> MRVEGAIGKTPVVRLAKVVEPDMAEVWVKLEGLNPGGSIKDRPAWYMIKDAEERGILRPGSGQVIVEPTSGNTGIGLAMIA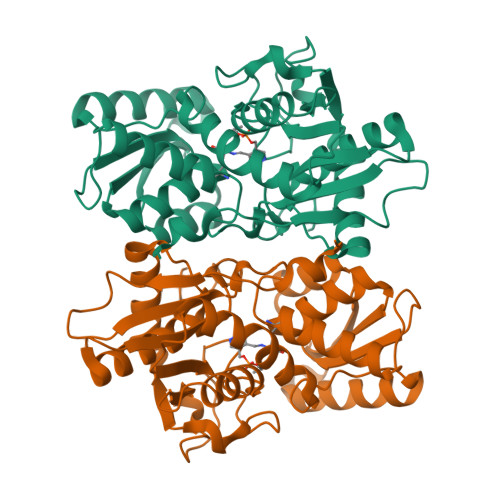ASRGYRLILTMPAQMSEERKRVLKAFGAELVLTDPERRMLAAREEALRLKEELGAFMPDQFKNPANVRAHYETTGPELYEALEGRIDAFVYGSGTGGTITGVGRYLKERIPHVKVIAVEPARSNVLSGGKMGQHGFQGMGPGFIPENLDLSLLDGVIQVWEEDAFPLARRLAREEGLFLGMSSGGIVWAALQVARELGPGKRVACISPDGGWKYLSTPLYAEP>[2x]MEEVKKDVYSVWALPDEESEPRFKKLMEALRSEFTGPRFVPHVTVAVSAYLTADEAKKMFESACDGLKAYTATVDRVSTGTFFFQCVFLLLQTTPEVMEAGEHCK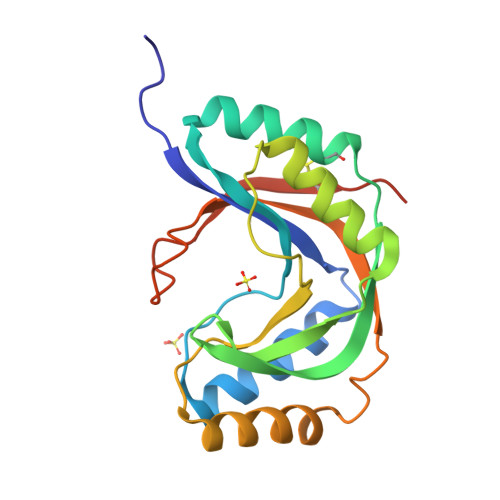NHFNCSTTTPYMPHLSLLYAELTEEEKKNAQEKAYTLDSSLDGLSFRLNRLALCKTDTEDKTLETWETVAVCNLNPGSHHHHHH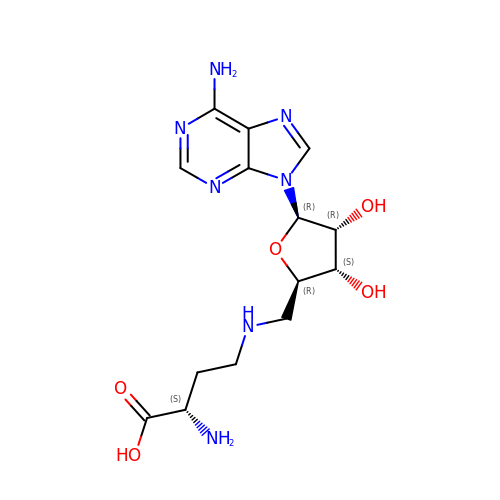5'-{[(3S)-3-amino-3-carboxypropyl]amino}-5'-deoxyadenosine | C14 H21 N7 O5 | WSOGVCAFRBSBRE-WFMPWKQPSA-N> VPTNTPTNTPANTPVSGNLKVEFYNSNPSDTTNSINPQFKVTNTGSSAIDLSKLTLRYYYTVDGQKDQTFWCDHAAIIGSNG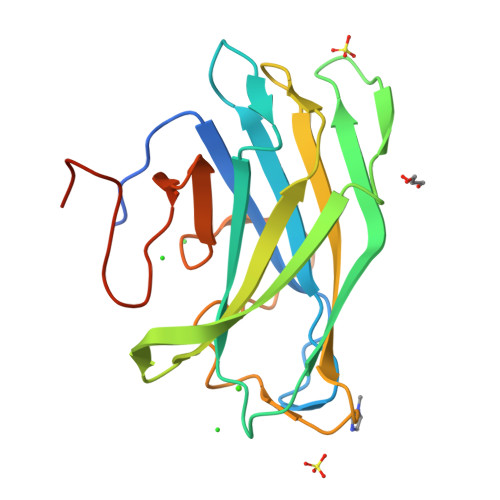SYNGITSNVKGTFVKMSSSTNNADTYLEISFTGGTLEPGAHVQIQGRFAKNDWSNYTQSNDYSFKSASQFVEWDQVTAYLNGVLVWGKEPGGSVVPSTQPVTTPPATT> MASSSHNPVILLKRILSLTESSPFILCLDSIAQTSYKLIQEFVHQSKSKGNEYPIVYISFETVNKPSYCTQFIDATQMDFVHLVKQIISYLPAATATQAKKHMVIIDSLNYISTEYITRFLSEIASPHCTMVATYHKDIKDENRTVIPDWNNNYPDKLTLLQFMATTIVDIDVVLTGTLDTEEVSELLNEFRIPRGLNNDIFQLRLVNKRKSGRS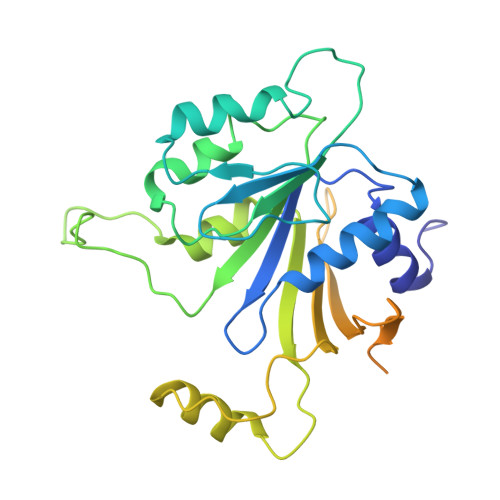LEYDFIVNSNTHEYELLSTTKQEEESSSNGLETPEMLQGLTTFNLGTSNKQKLAKDQVALPFLEAQSFGQGGAIVYEYEKDDDYDEEDPYEDPF>MGKAVIAIHGGAGAISRAQMSLQQELRYIEALSAIVETGQKMLEAGESALDVVTEAVRLLEECPLFNAGIGAVFTRDETHELDACVMDGNTLKAGAVAGVSHLRNPVLAARLVMEQSPHVMMIGEGAENFAFARGMERVSPEIFSTSLRYEQLLAARKEGATVLDHSGAPLDEKQKMG[2x];>TVGAVALDLDGNLAAATSTGGMTNKLPCTVGAAPLVGAGCYANNASVAVSCTGTGEVFIRALAAYDIAALMDYGGLSLAEACERVVMEKLPALGGSGGLIAIDHEGNVALPFNTEGMYRAWGYAGDTPTTGIYREKGDTVATQ[2x]

l-Asparaginases hydrolyze l-asparagine to l-aspartic acid and ammonia. The prototypic class 2 enzyme is EcAIII from E. coli. EcAIII belongs to the Ntn-hydrolases, which are expressed as immature polypeptides that dimerize and then autocatalytically cleave themselves into α (∼20 kDa) and β (∼15 kDa) subunits to form the mature (αβ)2 heterotetramer (a dimer of two αβ heterodimers). The same Thr179 acts as the nucleophile in the autoproteolytic maturation and in l-asparagine hydrolysis.

In mutant RDM1-12, Cys206 and Thr207 do not affect the neighboring residues. The D210A and S211A substitutions, located close to the threonine triad, despite the presence of two small nonpolar alanines, do not affect the conformation of the adjacent side chains but modify the pattern of hydrogen bonds to water molecules. The side chain of Glu234, rotated towards Arg238, has a slightly different conformation and a different pattern of hydrogen bonds in the two subunits. In other variants, for example RDM1-12, differences are visible in the regions of α-helix 147–159, loop 200–208 and loop 116–120, while in RDM1-38 differences are only observed in the region of α-helix 147–159. Moreover, a multi-step denaturation process was observed for most of them. Analysis of T m of the autoprocessing mutants reveled that they can be divided into two groups: those with decreased (RDM1-3, RDM1-8, RDM1-29 and RDM1-37) and increased (RDM1-12, RDM1-18, RDM1-24 and RDM1-38) T m values.> VKDLLKFLKAQTKTEEFDAIKIALASPDMIRSWSFGEVKKPETINYRTFKPERDGLFCARIFGPVKDYECLCGKYKRLKHRGVICEKCGVEVTQTKVRRERMGHIELASPTAHIWFLKSLPSRIGLLLDMPLRDIERVLYFESYVVIEGGMTNLERQQILTEEQYLDALEEFGDEFDAKMGAEAIQALLKSMDLEQECEQLREELNETNSETKRKKLTKRIKLLEAFVQSGNKPEWMILTVLPVLPPDLRPLVPLDGGRFATSDLNDLYRRVINRNNRLKRLLDLAAPDIIVRNEKRMLQEAVDALLDNGRRGRAITGSNKRPLKSLADMIKGKQGRFRQNLLGKRVDYSGRSVITVGPYLRLHQCGLPKKMALELFKPFIYGKLELRGLATTIKAAKKMVEREEAVVWDILDEVIREHPVLLNRAPTLHRLGIQAFEPVLIEGKAIQLHPLVCAAYNADFDGDQMAVHVPLTLEAQLEARALMMSTNNILSPANGEPIIVPSQDVVLGLYYMTRDCVNAKGEGMVLTGPKEAERLYRSGLASLHARVKVRITEYEKDANGELVAKTSLKDTTVGRAILWMIVPKGLPYSIVNQALGKKAISKMLNTCYRILGLKPTVIFADQIMYTGFAYAARSGASVGIDDMVIPEKKHEIISEAEAEVAEIQEQFQSGLVTAGERYNKVIDIWAAANDRVSKAMMDNLQTETVINRDGQEEKQVSFNSIYMMADSGARGSAAQIRQLAGMRGLMAKPDGSIIETPITANFREGLNVLQYFISTHGARKGLADTALKTANSGYLTRRLVDVAQDLVVTEDDCGTHEGIMMTPVIEGGDVKEPLRDRVLGRVTAEDVLKPGTADILVPRNTLLHEQWCDLLEENSVDAVKVRSVVSCDTDFGVCAHCYGRDLARGHIINKGEAIGVIAAQSIGEPGTQLTMRTFHIGGAASRAAAESSIQVKNKGSIKLSNVKSVVNSSGKLVITSRNTELKLIDEFGRTKESYKVPYGAVLAKGDGEQVAGGETVANWDPHTMPVITEVSGFVRFTDMIDGQTITRQTDELTGLSSLVVLDSAERTAGGKDLRPALKIVDAQGNDVLIPGTDMPAQYFLPGKAIVQLEDGVQISSGDTLARIPQESGGTKDITGGLPRVADLFEARRPKEPAILAEISGIVSFGKETKGKRRLVITPVDGSDPYEEMIPKWRQLNVFEGERVERGDVISDGPEAPHDILRLRG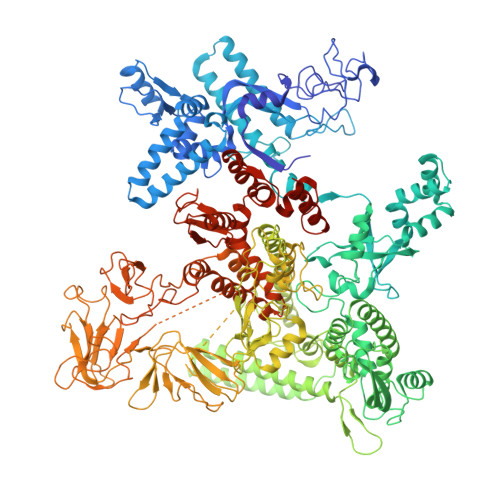VHAVTRYIVNEVQDVYRLQGVKINDKHIEVIVRQMLRKATIVNAGSSDFLEGEQVEYSRVKIANRELEANGKVGATYSRDLLGITKASLATESFISAASFQETTRVLTEAAVAGKRDELRGLKENVIVGRLIPAGTGYAYHQDRMRRRAAGEAPAAPQVTAEDASASLAELLNAGLGGSDNE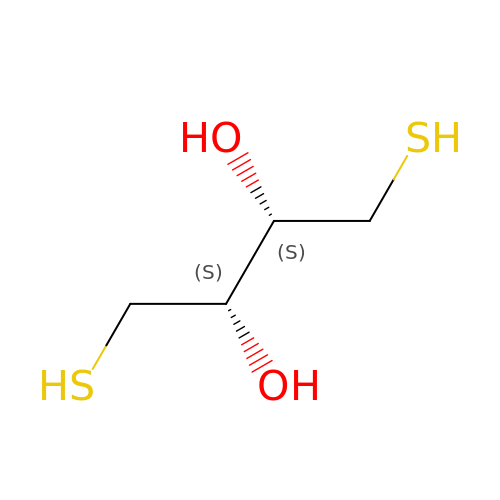(2S,3S)-1,4-DIMERCAPTOBUTANE-2,3-DIOL | C4 H10 O2 S2 | VHJLVAABSRFDPM-QWWZWVQMSA-N> GALDDLWADELGRTRMTIKELLRLTQGSVVALDGLAGEPLDILINGYLIAQGEVVVVADKYG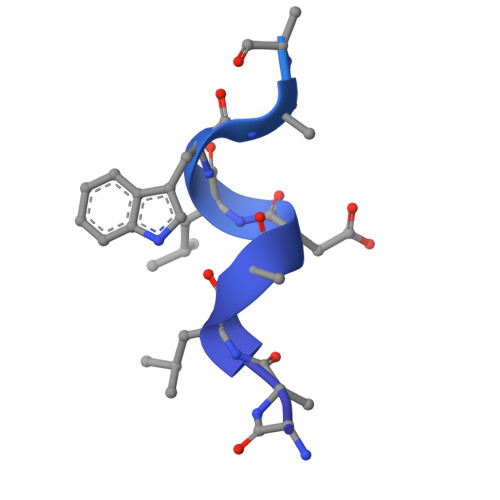VRITDIITPSERMRRLSR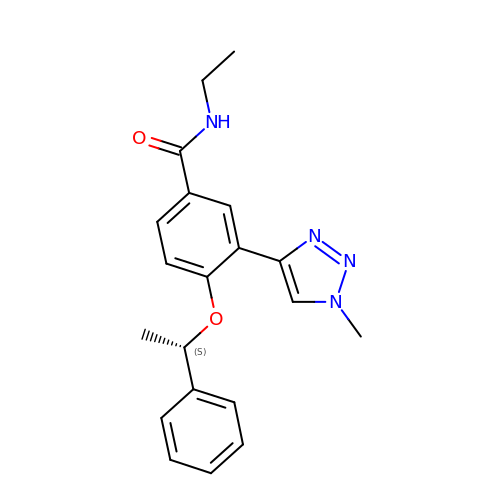~{N}-ethyl-3-(1-methyl-1,2,3-triazol-4-yl)-4-[(1~{S})-1-phenylethoxy]benzamide | C20 H22 N4 O2 | VZVLEUYPQRNNJB-AWEZNQCLSA-N>MSLGVTNRLACYSDPADHYSHRVRIVLAEKGVSAEIISVEAGRQPPKLIEVNPYGSLPTLVDRDLALWESTVVMEYLDERYPHPPLLPVYPVARANSRLLIHRIQRDWCGQVDLILDPRTKEAARVQARKELRESLTGVSPLFADKPFFLSEEQSLVDCCLLPILWRLPVLGIELPRQAKPLLDYMERQ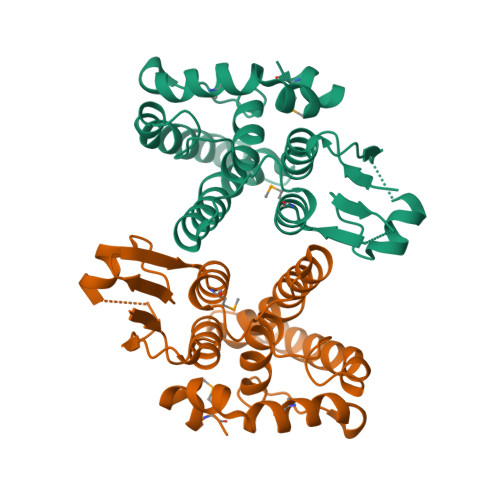FAREAFQASLSGVERDMREGHHHHHH[2x]> GNVLDFKWYTRKAESWGVQTFKNWKENLTISEKDIITGYTGSKYDPINEYLRKYDGEIIPNIGGDLDKKSKKALEKIENQIKNLDAALQKSKITENLIVYRRVSELQFGKKYEDYNLRQNGIINEEKVMELESNFKGQTFIQHNYMSTSLVQDPHQSYSNDRYPILLEITIPEGVHGAYIADMSEYPGQYEMLINRGYTFKYD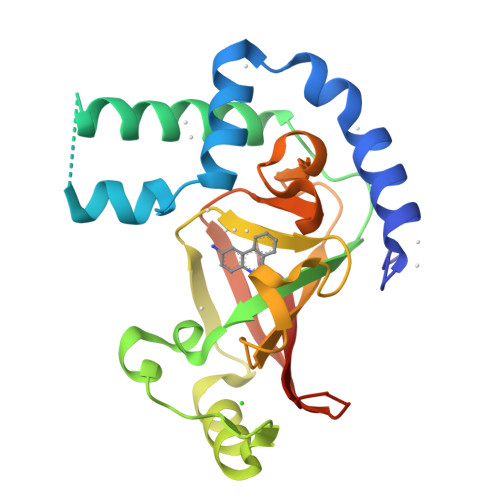KFSIVKPTREEDKGKEYLKVNLSIYL> GPAMDGTAAEPRPGAGSLQHAQPPPQPRKKRPEDFKFGKILGEGSFSTVVLARELATSREYAIKILEKRHIIKENKVPYVTRERDVMSRLDHPFFVKLYFTFQDDEKLYFGLSYAKNGELLKYIRKIGSFDETCTRFYTAEIVSALEYLHGKGIIHRDLKPENILLNEDMHIQITDFGTAKVLSPESKQARANSFVGTA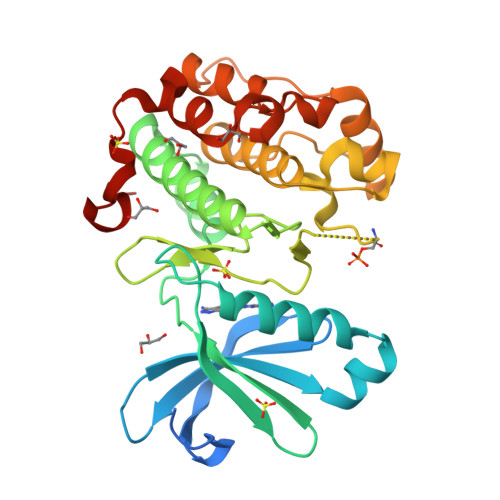QYVSPELLTEKSACKSSDLWALGCIIYQLVAGLPPFRAGNEYLIFQKIIKLEYDFPEKFFPKARDLVEKLLVLDATKRLGCEEMEGYGPLKAHPFFESVTWENLHQQTPPKLT> GSNFAILPSLQQFNKVLAYE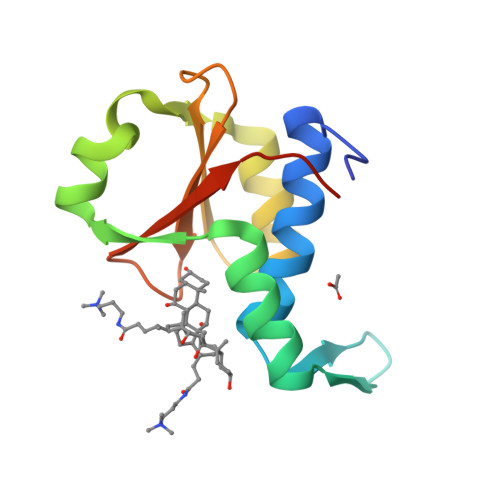VRMLMTDKLQLEDGTQLVVPPAFRREIYRELGISLYSNEAAEEAGLRWAQHYEFLSHQMAQQLGGPTEVRVEVNKSSPVVWLKTWLSPNIWVRVPLTEIHQGDFS> STRDYEIQRERIELGRCIGEGQFGDVHQGIYMSPENPAMAVAIKTCKNCTSDSVREKFLQEALTMRQFDHPHIVKLIGVITENPVWIIMELCTLGELRSFLQVRKFSLDLASLILYAYQLSTALAYLESKRFVHRDIAARNVLVSATDCVKLGDFGLSRYMEDSTYYKASKGKLPIKWMAPESINFRRFTSASDVWMFGVCMWEILMHGVK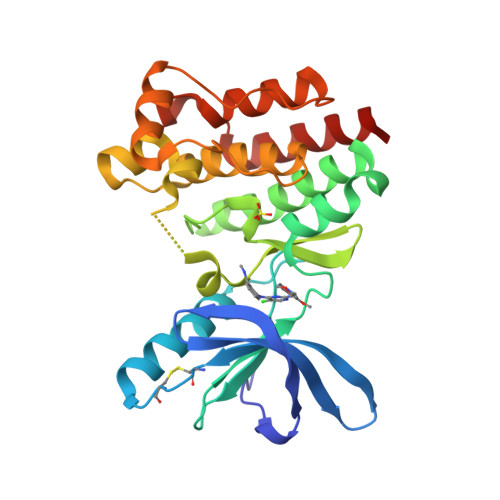PFQGVKNNDVIGRIENGERLPMPPNCPPTLYSLMTKCWAYDPSRRPRFTELKAQLSTILEEEKLQ>MWSHPQFEKASMVLMIVSGRSGSGKSVALRALEDMGFYCVDNLPVVLLPDLARTLADREISAAVSIDVRNMPESPEIFEQAMSNLPDAFSPQLLFLDADRNTLIRRYSDTRRLHPLSSKNLSLESAIDKESDLLEPLRSRADLIVDTSEMSVHELAEMLRTRLLGKRERELTMVFESFGFKHGIPIDADYVFDVRFLPNPHWDPKLRPMTGLDKPVAAFLDRHTEVHNFI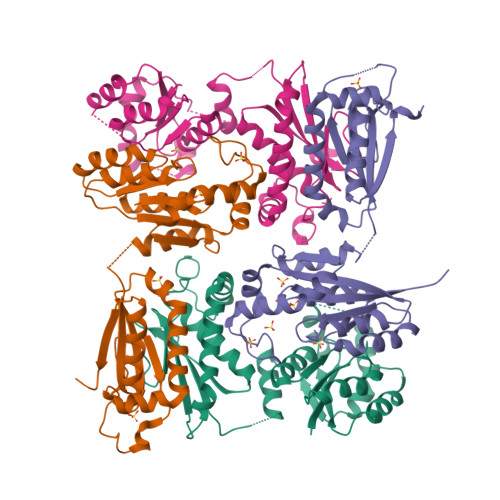YQTRSYLELWLPMLETNNRSYLTVAIGCTGGKHRSVYIAEQLADYFRSRGKNVQSRHRTLEKRKP[4x]Copper-containing nitrite reductases (CuNIRs) catalyze transformation of nitrite to nitric oxide, which has impacts on geochemical, agricultural, and medical health fields. CuNIRs typically have an ∼110 kDa homotrimeric structure, like a Reuleaux triangle. Each protomer contains one type 1 copper (T1Cu) and one type 2 copper (T2Cu) site. The Cys residue forms a peptide-bond bridge (Cys-His bridge) together with one of the His ligands at the T2Cu site to transfer the electron to the catalytic T2Cu site, which is coordinated by three His residues and an axial water molecule.

Since the GK-like conformer complicates the interpretation of the T2Cu site structure, we constructed D98N/G136A and D98N/C135A/G136A mutants. We expected that replacing Gly136 with alanine would cause steric hindrance between the side chain methyl group of Ala136 and the GK-like state of Asn98. The structures of D98N/G136A without NO2- and D98N/C135A/G136A in complex with NO2- were determined at 0.96 and 0.99 Å resolution, respectively. These sub-ångström resolution data depict H atom positions on Asn98 and HisCAT, although the H atom positions of BW were ambiguous. The two H atoms of the Asn98 side chain are not on the carbamoyl plane but rather are oriented toward the ligand molecule on the T2Cu atom. This indicates that Asn98 (and perhaps also protonated Asp98) forms an H-bond with the T2Cu axial ligand. As was expected, Asn98 does not exhibit the GK-like conformation in either of the G136A-containing mutants.

> NVIAAHKGVNQAPVPLKMERVGPHDVHIEMTAQITDIEIDKGKIYKAWTFNGQAPGPLVVVNEGDTIHFTLKNMDPVVPHSMNFHAVHASPSKDFIDVMPNKSGTFTYPANKPGVFMYHCATKPVLQHIANGMHGVIIVKPKNGYPTDKEVDREYVLIQNEWYKYNDMNDFQNGVPSYVVFSSKALKPGDPNTNGDTFTLKEKPLLAKVGEKIRLYINNVGPNEVSSFHVVGTVFDDVYLDGNPNNHLQGMQTVMLPASGGAVVEFTVTRPGTYPIVTHQFNHAQKGAVAMLKVTETGED> MATLFIADLHLQTEEPAITAGFLRFLQGEARQADALYILGDLFEAWIGDDDPNPLHQQIASAIKAVVDAGVPCYFIHGNRDFLVGQRFARQSGMILLAEEERLDLYGREVLIMHGDTLCTDDQGYLAFRAKVHTPWIQRLFLALPLFIRHRIAARMRADSKAANSSKSMEIMDVNPQAVVDAME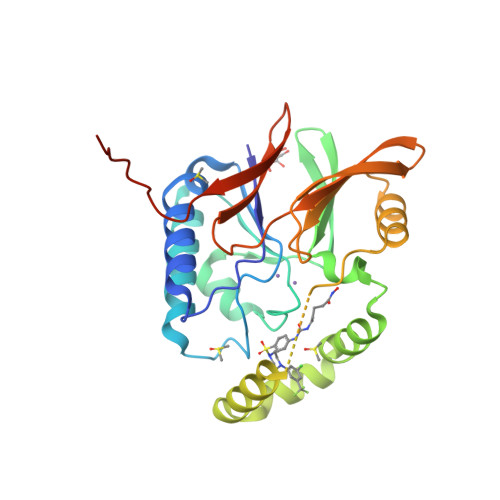RHHVQWLIHGHTHRPAVHELQANGQPAWRVVLGAWHSEGSMVKVTPDDVELIHFPFLEENLYFQSHHHHHHHHHH> LIQERRSHE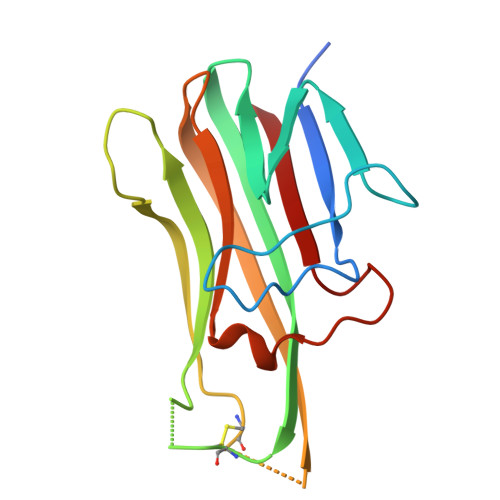VNPAAHLTGANSSLTGSGGPLLWETQLGLAFLRGLSYHDGALVVTKAGYYYIYSKVQLGGVGCPLGLASTITHGLYKRTPRYPEELELLVSQQSPCGRATSSSSNWFDSSFLGGVVHLEAGEEVVVRVLDERLVRLRDGTRSYFGAFMV> MIPAALPHPTMKRQGDRDIVVTGVRNQFATDLEPGGSVSCMRSSLSFLSLLFDVGPRDVLSAEAIEGCLVEGGEWTRAAAGSGPPRMCSIIELPNFLEYPAARGGLRCVFSRVYGEVGFFGEPTAGLLETQCPAHTFFAGPWAMRPLSYTLLTIGPLGMGLYRDGDTAYLFDPHGLPAGTPAFIAKVRAGDVYPYLTYYAHDRPKVRWAGAMVFFVPSGPGAVAPADLTAAALHLYGASETYLQDEPFVERRVAITHPLRGEIGGLGALFVGVVPRGDGEGSGPVVPALPAPTHVQTPGADRPPEAPRGASGPPDTPQAGHPNRPPDDVWAAALEGTPPAKPSAPDAAASGPPHAAPPPQTPAGDAAEEAEDLRVLEVGAVPVGRHRARYSTGLPKRRRPTWTPPSSVEDLTSGERPAPKAPPAKAKKKSAPKKKAPVAAEVPASSPTPIAATVPPAPDTPPQSGQGGGDDGPASPSSPSVLETLGARRPPEPPGADLAQLFEVHPNVAATAVRLAARDAALAREVAACSQLTINALRSPYPAHPGLLELCVIFFFERVLAFLIENGARTHTQAGVAGPAAALLDFTLRMLPRKTAVGDFLASTRMSLADVAAHRPLIQHVLDENSQIGRLALAKLVLVARDVIRETDAFYGDLADLDLQLRAAPPANLYARLGEWLLERSRAHPNTLFAPATPTHPEPLLHRIQALAQFARGEEMRVEAEAREMREALDALARGVDSVSQRAGPLTVMPVPAAPGAGGRAPCPPALGPEAIQARLEDVRIQARRAIESAVKEYFHRGAVYSAKALQASDSHDCRFHVASAAVVPMVQLLESLPAFDQHTRDVAQRAALPPPPPLATSPQAILLRDLLQRGQPLDAPEDLAAWLSVLTDAATQGLIERKPLEELARSIHGINDQQARRSSGLAELQRFDALDAALAQQLDSDAAFVPATGPAPYVDGGGLSPEATRMAEDALRQARAMEAAKMTAELAPEARSRLRERAHALEAMLNDARERAKVAHDAREKFLHKLQGVLRPLPDFVGLKACPAVLATLRASLPAGWTDLADAVRGPPPEVTAALRADLWGLLGQYREALEHPTPDTATALAGLHPAFVVVLKTLFADAPETPVLVQFFSDHAPTIAKAVSNAINAGSAAVATASPAATVDAAVRAHGALADAVSALGAAARDPASPLSFLAVLADSAAGYVKATRLALEARGAIDELTTLGSAAADLVVQARRACAQPEGDHAALIDAAARATTAARESLAGHEAGFGGLLHAEGTAGDHSPSGRALQELGKVIGATRRRADELEAAVADLTAKMAAQ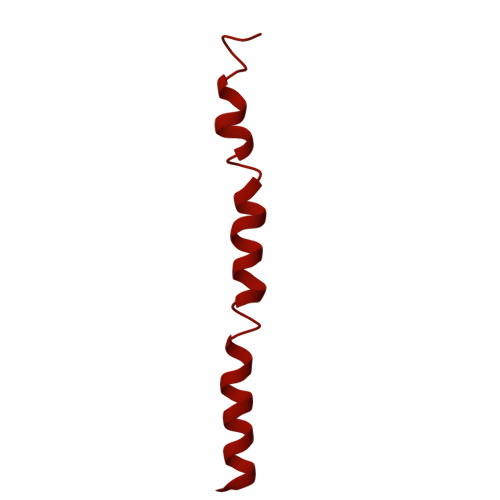RARGSSERWAAGVEAALDRVENRAEFDVVELRRLQALAGTHGYNPRDFRKRAEQALAANAEAVTLALDTAFAFNPYTPENQRHPMLPPLAAIHRLGWSAAFHAAAETYADMFRVDAEPLARLLRIAEGLLEMAQAGDGFIDYHEAVGRLADDMTSVPGLRRYVPFFQHGYADYVELRDRLDAIRADVHRALGGVPLDLAAAAEQISAARNDPEATAELVRTGVTLPCPSEDALVACAAALERVDQSPVKNTAYAEYVAFVTRQDTAETKDAVVRAKQQRAEATERVMAGLREALAARERRAQIEAEGLANLKTMLKVVAVPATVAKTLDQARSVAEIADQVEVLLDQTEKTRELDVPAVIWLEHAQRTFETHPLSAARGDGPGPLARHAGRLGALFDTRRRVDALRRSLEEAEAEWDEVWGRFGRVRGGAWKSPEGFRAMHEQLRALQDTTNTVSGLRAQPAYERLSARYQGVLGAKGAERAEAVEELGARVTKHTALCARLRDEVVRRVPWEMNFDALGGLLAEFDAAAADLAPWAVEEFRGARELIQYRMGLYSAYARAGGQTGAGAESAPAPLLVDLRALDARARASSSPEGHEVDPQLLRRRGEAYLRAGGDPGPLVLREAVSALDLPFATSFLAPDGTPLQYALCFPAVTDKLGALLMRPEAACVRPPLPTDVLESAPTVTAMYVLTVVNRLQLALSDAQAANFQLFGRFVRHRQATWGASMDAAAELYVALVATTLTREFGCRWAQLGWASGAAAPRPPPGPRGSQRHCVAFNENDVLVALVAGVPEHIYNFWRLDLVRQHEYMHLTLERAFEDAAESMLFVQRLTPHPDARIRVLPTFLDGGPPTRGLLFGTRLADWRRGKLSETDPLAPWRSALELGTQRRDVPALGKLSPAQALAAVSVLGRMCLPSAALAALWTCMFPDDYTEYDSFDALLAARLESGQTLGPAGGREASLPEAPHALYRPTGQHVAVLAAATHRTPAARVTAMDLVLAAVLLGAPVVVALRNTTAFSRESELELCLTLFDSRPGGPDAALRDVVSSDIETWAVGLLHTDLNPIENACLAAQLPRLSALIAERPLADGPPCLVLVDISMTPVAVLWEAPEPPGPPDVRFVGSEATEELPFVATAGDVLAASAADADPFFARAILGRPFDASLLTGELFPGHPVYQRPLADEAGPSAPTAARDPRDLAGGDGGSGPEDPAAPPARQADPGVLAPTLLTDATTGEPVPPRMWAWIHGLEELASDDAGGPTPNPAPALLPPPATDQSVPTSQYAPRPIGPAATARETRPSVPPQQNTGRVPVAPRDDPRPSPPTPSPPADAALPPPAFSGSAAAFSAAVPRVRRSRRTRAKSRAPRASAPPEGWRPPALPAPVAPVAASARPPDQPPTPESAPPAWVSALPLPPGPASARGAFPAPTLAPIPPPPAEGAVVPGGDRRRGRRQTTAGPSPTPPRGPAAGPPRRLTRPAVASLSASLNSLPSPRDPADHAAAVSAAAAAVPPSPGLAPPTSAVQTSPPPLAPGPVAPSEPLCGWVVPGGPVARRPPPQSPATKPAARTRIRARSVPQPPLPQPPLPQPPLPQPPLPQPPLPQPPLPQPPLPQPPLPQPPLPQPPLPQPPLPPVTRTLTPQSRDSVPTPESPTHTNTHLPVSAVTSWASSLALHVDSAPPPASLLQTLHISSDDEHSDADSLRFSDSDDTEALDPLPPEPHLPPADEPPGPLAADHLQSPHSQFGPLPVQANAVLSRRYVRSTGRSALAVLIRACRRIQQQLQRTRRALFQRSNAVLTSLHHVRMLLG>MSEITIGVLSLQGDFEPHINHFIKLQIPSLNIIQVRNVHDLGLCDGLVIPGGESTTVRRCCAYENDTLYNALVHFIHVLKKPIWGTCAGCILLSKNVENIKLYSNFGNKFSFGGLDITICRNFYGSQNDSFICSLNIISDSSAFKKDLTAACIRAPYIREILSDEVKVLATFSHESYGPNIIAAVEQNNCLGTVFHPELLPHTAFQQYFYEKV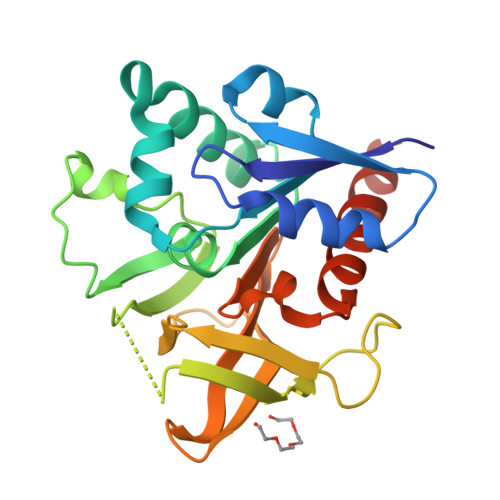KNYKYSLEHHHHHH[2x]> KETAAAKFERQHMDSSTSAASSSNYCNQMMKSRNLT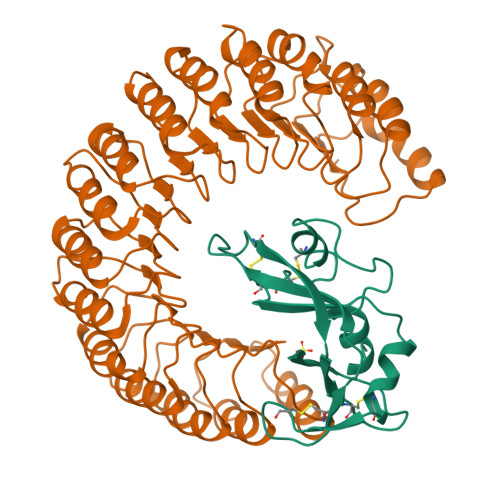KDRCKPVNTFVHESLADVQAVCSQKNVACKNGQTNCYQSYSTMSITDCRETGSSKYPNCAYKTTQANKHIIVACEGNPYVPVHFDASV;> XMNLDIHCEQLSDARWTELLPLLQQYEVVRLDDCGLTEEHCKDIGSALRANPSLTELCLRTNELGDAGVHLVLQGLQSPTCKIQKLSLQNCSLTEAGCGVLPSTLRSLPTLRELHLSDNPLGDAGLRLLCEGLLDPQCHLEKLQLEYCRLTAASCEPLASVLRATRALKELTVSNNDIGEAGARVLGQGLADSACQLETLRLENCGLTPANCKDLCGIVASQASLRELDLGSNGLGDAGIAELCPGLLSPASRLKTLWLWECDITASGCRDLCRVLQAKETLKELSLAGNKLGDEGARLLCESLLQPGCQLESLWVKSCSLTAACCQHVSLMLTQNKHLLELQLSSNKLGDSGIQELCQALSQPGTTLRVLCLGDCEVTNSGCSSLASLLLANRSLRELDLSNNCVGDPGVLQLLGSLEQPGCALEQLVLYDTYWTEEVEDRLQALEGSKPGLRVIS>DVTQVAQIMNTNPVSITADKSLQAAITVMKEKRVDTLLVVDEGNVLKGFIDVEQIDLNRRTATSVMDIIEKNVFYVYED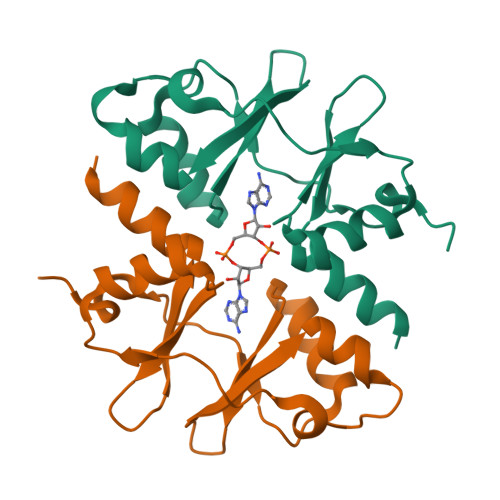TLLRDTVQRILKRGYKYIPVVDKDKRLVGIVTRASLVDIVYDSIWGT[2x]> MKSSDIFHACKYTPILLKSRTNDSGVNQYGLRPVNSYDYLNPTNLVNFGRGTAFDNLGVRRSERGQIDSAPSLGGSPVFTQAKLLGLSGDDQLRLCEAETTQLRMCMAKGGSACERESLLLDACLSKVGHLRRAISQAGSEFNDWFIQNVSDNHTKPFQHRPHDWRHYYAQEKLVREKQQNGHAYGRRPKEFSF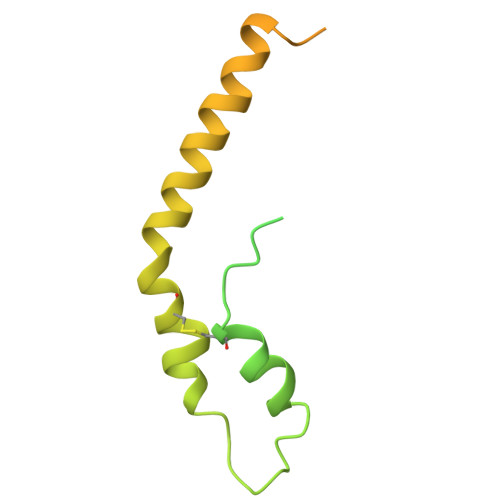GARYVKTEGYGKRPRLPYNK> SNAMEELTLKGVTQYYAYVTERQKVHCLNTLFSRLQINQSIIFCNSSQRVELLAKKISQLGYSCFYIHAKMRQEHRNRVFHDFRNGLCRNLVCTDLFTRGIDIQAVNVVI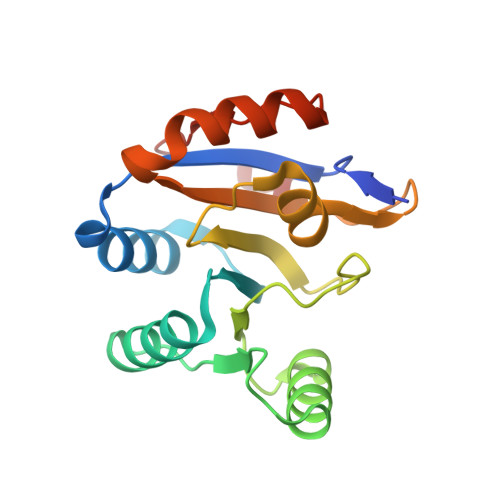NFDFPKLAETYLHRIGRSGRFGHLGLAINLITYDDRFNLKSIEEQLGTEIKPIPSNIDKSLY> 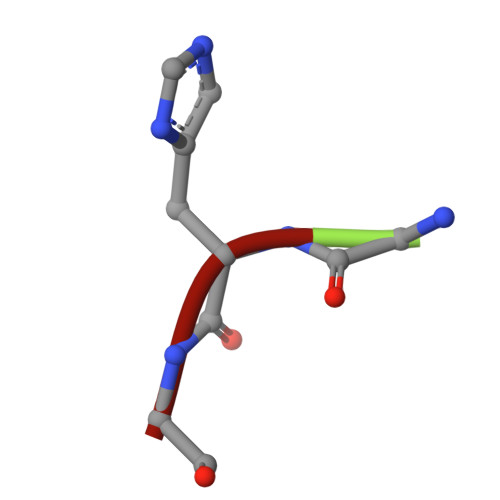GHG>[2x]MVDPQLDGPQLAALAAVVELGSF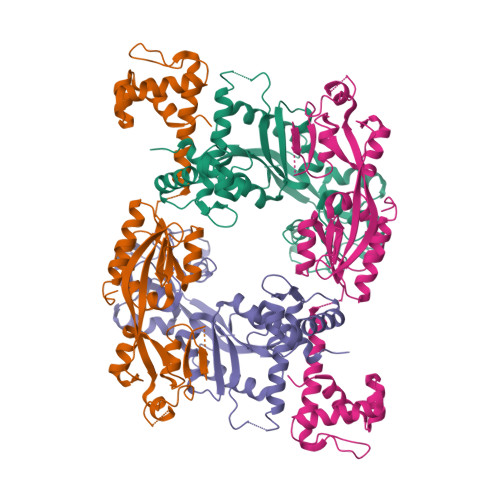DAAAERLHVTPSAVSQRIKSLEQQVGQVLVVREKPCRATTAGIPLLRLAAQTALLESEALAEMGGNASLKRTRITIAVNADSMATWFSAVFDGLGDVLLDVRIEDQDHSARLLREGVAMGAVTTERNPVPGCRVHPLGEMRYLPVASRPFVQRHLSDGFTAAAAAKAPSLAWNRDDGLQDMLVRKAFRRAITRPTHFVPTTEGFTAAARAGLGWGMFPEKLAASPLADGSFVRVCDIHLDVPLYWQCWKLDSPIIARITDTVRAAASGLYRGQQRRRRPG> GLGYGSWEIDPKDLTFLKELGTGQFGVVKYGKWRGQYDVAIKMIKEGSMSEDEFIEEAKVMMNLSHEKLVQLYGVCTKQRPIFI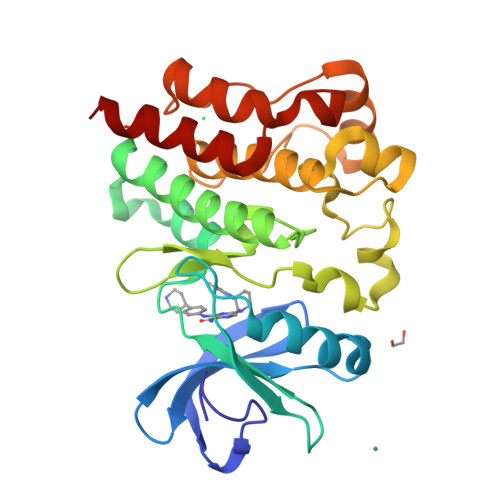ITEYMANGCLLNYLREMRHRFQTQQLLEMCKDVCEAMEYLESKQFLHRDLAARNCLVNDQGVVKVSDFGLSRYVLDDEYTSSVGSKFPVRWSPPEVLMYSKFSSKSDIWAFGVLMWEIYSLGKMPYERFTNSETAEHIAQGLRLYRPHLASEKVYTIMYSCWHEKADERPTFKILLSNILDVMDEE>MSASKILSQKIKVALVQLSGSSPDKMANLQRAATFIERAMKEQPDTKLVVLPECFNSPYSTDQFRKYS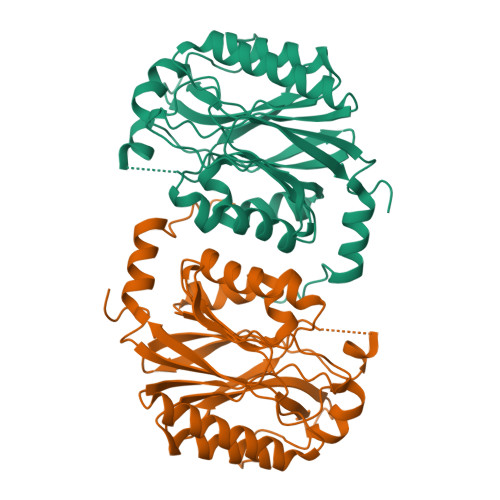EVINPKEPSTSVQFLSNLANKFKIILVGGTIPELDPKTDKIYNTSIIFNEDGKLIDKHRKVHLFDVDIPNGISFHESETLSPGEKSTTIDTKYGKFGVGICYDMRFPELAMLSARKGAFAMIYPSAFNTVTGPLHWHLLARSRAVDNQVYVMLCSPARNLQSSYHAYGHSIVVDPRGKIVAEAGEGEEIIYAELDPEVIESFRQAVPLTKQRRFDVYSDVNAH[2x]> K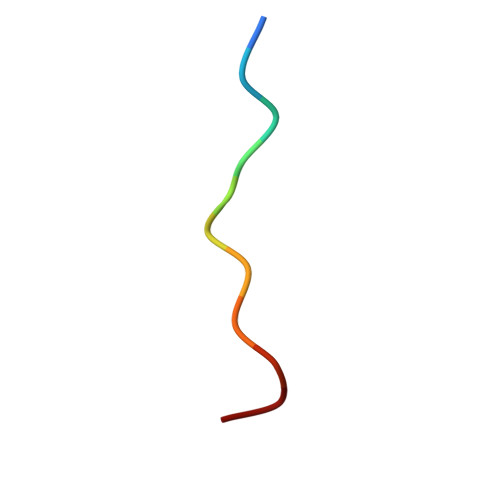STGGKAPRKQ>VKFDGVRPTRVEVYLDAITHNFREIKKIVGKNVKIMAVIKGDAYGHGASYVAKFLEKEGVDYFGVATTEEALELREKGIKTPILIFGYTPPTQLRQIVKHDLTQTVYDIKYAKELEKESLKQNKRAKVHIKIDTGLGRIGYIDFDLAQKEILEMANMRGLILEGIYSHFAAASEDDRDYCKEQFDKFMNLISSLEKKRLKIPLKHIANAAAILNLNYSHLDMVRPGIILFGAYPSKRVERKVELRETLRFTTRVVHLKDVPAGFFIGYGKSFVTKRKSVIATIPVGYADGLDRRLSNNYKLLLKGKYVPIVGRVCMDQCMIDVTDVEGVEIGDEVVIIGTQNNETVSVESMAD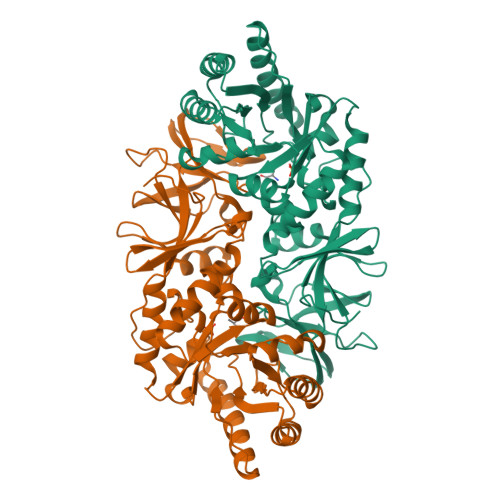KIETIPQEVFSRISRRVPRVYFYDGIKIGEVNYLK[2x]>[6x]SVGTFSLPALPYAYDALEPSISAQIMELHHSKHHQTYVTNLNNALKTYSTALAANDVPSQIALQAAIKFNGGGIINHSL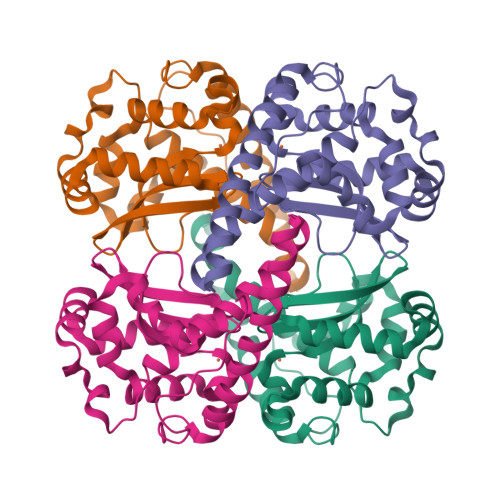FWENLCPASSPDADPASAPELTAEIAKTWGSLDKFKEAMGKALLGIQGSGWGWLVKEGSGLRIVTTKDQDPVVGGEVPVFGIDMWEHAYYLQYLNGKAAYVDNIWKVINWKTAEQRFKGDREDAFKILKASL6-amino-4-{2-[(cyclohexylmethyl)amino]ethyl}-2-(methylamino)-1,7-dihydro-8H-imidazo[4,5-g]quinazolin-8-one | C19 H27 N7 O | 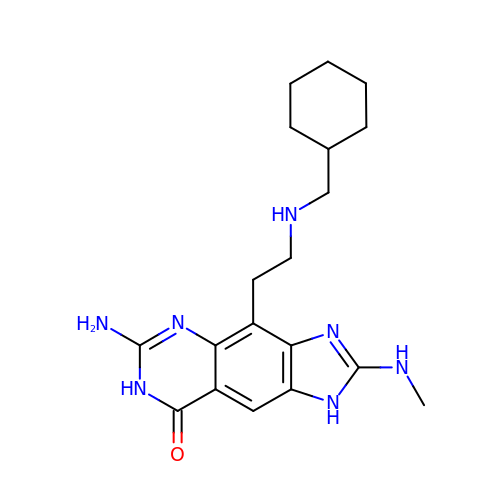ZKRVOXSNLYAMLM-UHFFFAOYSA-N> MPVAGSELPRRPLPPAAQERDAEPRPPHGELQYLGQIQHILRCGVRKDDRTGTGTLSVFGMQARYSLRDEFPLLTTKRVFW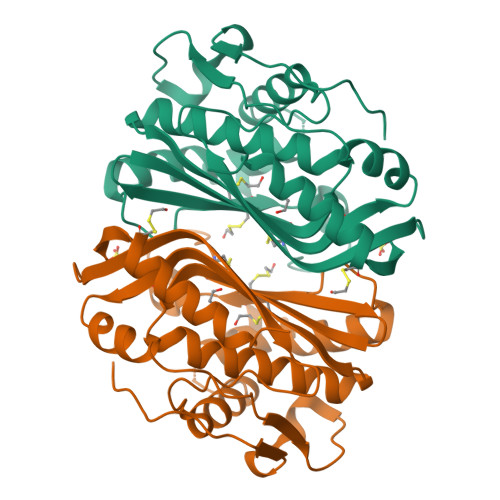KGVLEELLWFIKGSTNAKELSSKGVKIWDANGSRDFLDSLGFSTREEGDLGPVYGFQWRHFGAEYRDMESDYSGQGVDQLQRVIDTIKTNPDDRRIIMCAWNPRDLPLMKLPPCHALCQFYVVNSELSCQLYQRSGDMGLGVPFNIASYALLTYMIAHITGLKPGDFIHTLGDAHIYLNHIEPLKIQLQREPRPFPKLRILRKVEKIDDFKAEDFQIEGYNPHPTIKMEMAV> ETQPQMFFGVLDREELEYFKQAESTLQLDAFEAPEEKFQFVTSIIEEAKGKELKLVTSQITSKLMERVILECDETQLKDIFQSFNGVFFGLSCHKYASHVLETLFVRSAALVERELLTSGSVTMENMFLFMLNELKPHLKTMMNHQYASHVLRLLILILSSKTLPNSTKANSTLRSKKSKIARKMIDIKDNDDFNKVYQTPESFKSELRDIITTLYKGFTNGAESRSDISQSTITKFREYSVDKVASPVIQLIIQVEGIFDRDRSFWRLVFNTADEKDPKEESFLEYLLSDPVGSHFLENVIGSARLKYVERLYRLYMKDRIVKLAKRDTTGAFVVRALLEHLKEKDVKQILDAVVPELSML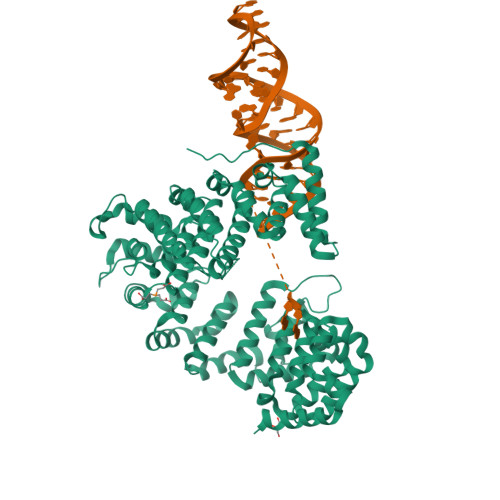LNSNMDFGTAIINTSNKQGGYLRDDVIAQLIQKYYPEKSDAKNILESCLLLSASTLGNTRDDWPTAEERRRSVFLEQLIDYDDKFLNITIDSMLALPEERLIQMCYHGVFSHVVEHVLQTTRVDIIKRKMLLNILSKESVNLACNVYGSHIMDKLWEFTAKLTLYKERIARALVLETEKVKNSIYGRQVWKNWKLELYVRKMWDWKKLIKEQEFEIFPNSKPLQPKPEK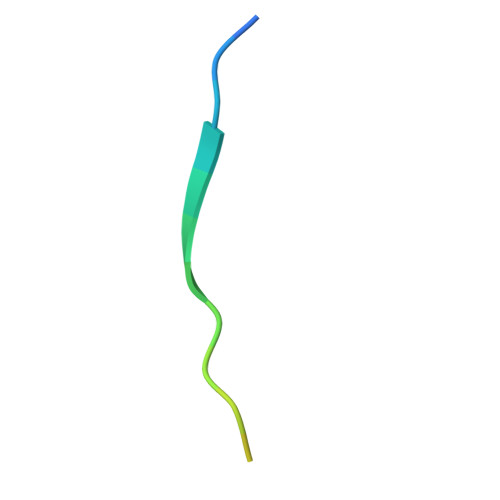> KEPSILIDVPLYQADTNDYLD2-(3-fluoro-2-methylbenzyl)-4-methyl-1-phenyl-3-(piperazin-1-ylcarbonyl)-1H-indol-5-ol | C28 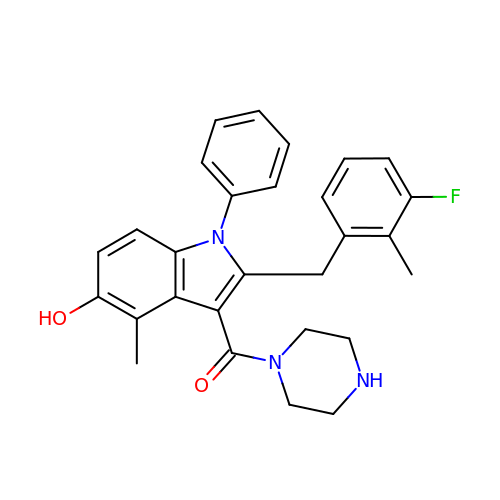H28 F N3 O2 | LWFGTVRNQYOUHL-UHFFFAOYSA-N>[2x]MSNKCDVVVVGGGISGMAAAKLLHDSGLNVVVLEARDRVGGRTYTLRNQKVKYVDLGGSYVGPTQNRILRLAKELGLETYKVNEVERLIHHVKGKSYPFRGPFPPVWNPITYLDHNNFWRTMDDMGREIPSDAPWKAPLAEEWDNMTMKELLDKLCWTESAKQLAT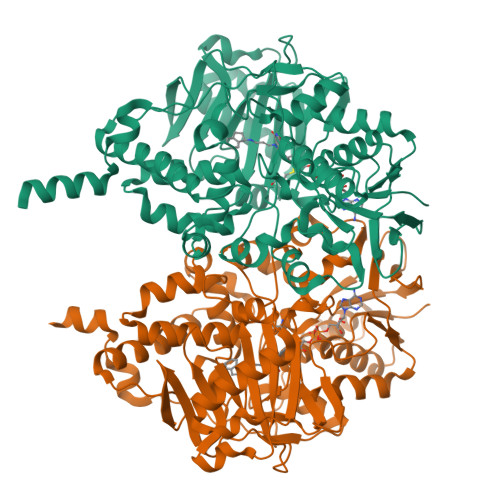LFVNLCVTAETHEVSALWFLWYVKQCGGTTRIISTTNGGQERKFVGGSGQVSERIMDLLGDRVKLERPVIYIDQTRENVLVETLNHEMYEAKYVISAIPPTLGMKIHFNPPLPMMRNQMITRVPLGSVIKCIVYYKEPFWRKKDYCGTMIIDGEEAPVAYTLDDTKPEGNYAAIMGFILAHKARKLARLTKEERLKKLCELYAKVLGSLEALEPVHYEEKNWCEEQYSGGCYTTYFPPGILTQYGRVLRQPVDRIYFAGTETATHWSGLMEGAVEAGERAAREILHAMGKIPEDEIWQSEPESVDVPAQPITTTFLERHLPSVPGLLRLIGLTTIFSATALGFLAHKRGLLVRV>MSSSGTPDLPVLLTDLKIQYTKIFINNEWHDSVSGKKFPVFNPATEEELCQVEEGDKEDVDKAVKAARQAFQIGSPWRTMDASERGRLLYKLADLIERDRLLLATMESMNGGKLYSNAYLSDLAGCIKTLRYCAGWADKIQGRTIPIDGNFFTYTRHEPIGVCGQIIPWNFPLVMLIWKIGPALSCGNTVVVKPAEQTPLTALHVASLIKEAGFPPGVVNIVPGYGPTAGAAISSHMDIDKVAFTGSTEVGKLIKEAAGKSNLKRVTLELGGKSPCIVLADADLDNAVEFAHHGVFYHQGQCCIAASRIFVEESIYDEFVRRSVERAKKYILGNPLTP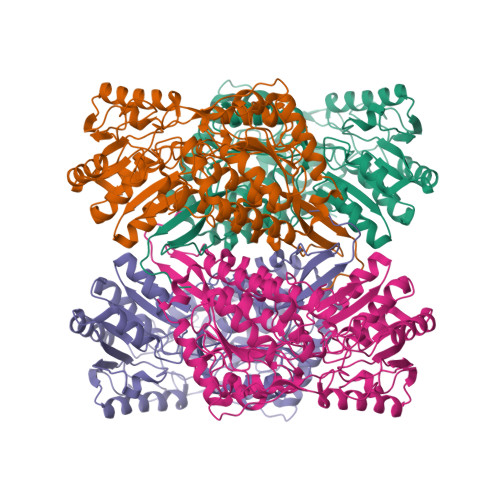GVTQGPQIDKEQYDKILDLIESGKKEGAKLECGGGPWGNKGYFVQPTVFSNVTDEMRIAKEEIFGPVQQIMKFKSLDDVIKRANNTFYGLSAGVFTKDIDKAITISSALQAGTVWVNCYGVVSAQCPFGGFKMSGNGRELGEYGFHEYTEVKTVTVKISQKNS[4x]>PPYTIVYFPVRGRCEAMRMLLADQGQSWKEEVVTIDTWMQGLLKPTCLYGQLPKFEDGDLTLYQSNAILRHLGRSLGLYGKNQREAAQMDMVNDGVEDLRGKYVTLIYTNYENGKNDYVKALPGHLKPFETLLSQNQGGKAFIVGDQISFADYNLLDLLLIHQVLAPGALDNFPLLSAYVARLSARPKIKAFL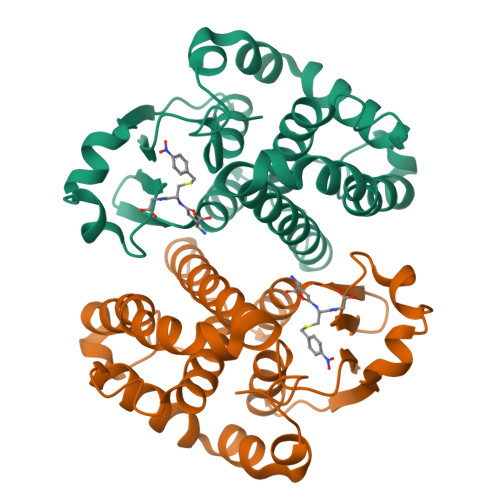SSPEHVNRPINGNGKQ[2x]>MEIRTFLERALKEDLGHGDLFERVLEKDFKATAFVRAKQEGVFSGEKYALELLEMTGIECVQTIKDKERFKPKDALMEIRGDFSMLLKVERTLLNLLQHSSGIATLTSRFVEALNSHKVRLLDT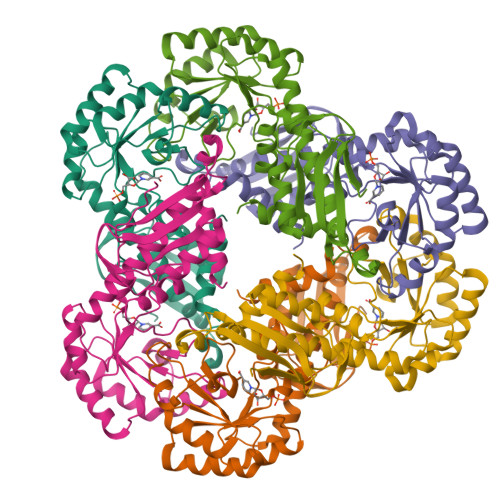RKTRPLLRIFEKYSVLNGGASNHRLGLDDALMLKDTHLRHVKDLKSFLTHARKNLPFTAKIEIECESFEEAKNAMNAGADIVMCDNLSVLETKEIAAYRDAHYPFVLLEASGNISLESINAYAKSGVDAISVGALIHQATFIDMHMKMA[3x]>[2x]PHMPPLPPGWEEKVDNLGRTYYV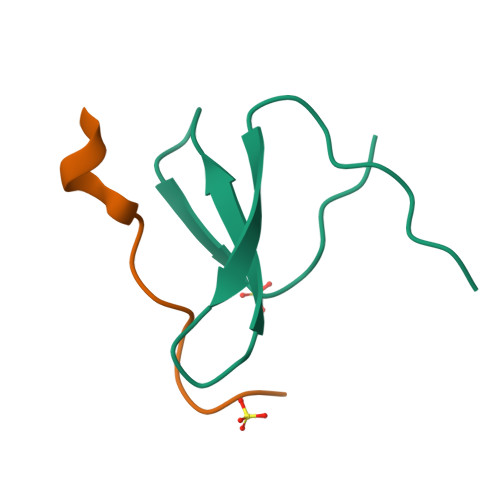NHNNRTTQWHRPSL;>EHRGPPPEYPFKGM[2x]> MNPVKREIHPDAVFYKEHKLRNDGLVITTNQGNIRLQFKSEAAIEVLYRADSKQLPSFALAQPESAIKAQLTETENHLQFSGGTLTARIQKRPFAISYYRDSELLLAEESGFQVNTDKINFRFYLSPGEKILGGGQRILGMDRRGQRFPLYNRAHYGYSDHSGQMYFGLPAIMSSKQYILVFDNSASGAMDIGKTESDILQLEAKSGRSAYILVAGNSYPSLIENFTQVTGRQPLPPRWALGSFASRFGYRSEAETRATVQKYKTEDFPLDTIVLDLYWFGKDIKGHMGNLDWDKENFPTPLDMMADFKQQGVKTVLITEPFVLTSSKRWDDAVKAKALAKDPQGQPKAFELYFGNGGIIDVFSKEGSRWFSSIYKDLSKQGVAGWWGDLGEPEMHPEDTQHAIGDADTVHNAYGHRWAEMLYQQQLDQFPELRPFIMMRAGFVGSQRYGMIPWTGDVSRTWGGLASQVELALQMSLLGFGYIHSDLGGFADGETLDKEMYIRWLQYGVFQPVYRPHGQDHIPSEPVFQDEE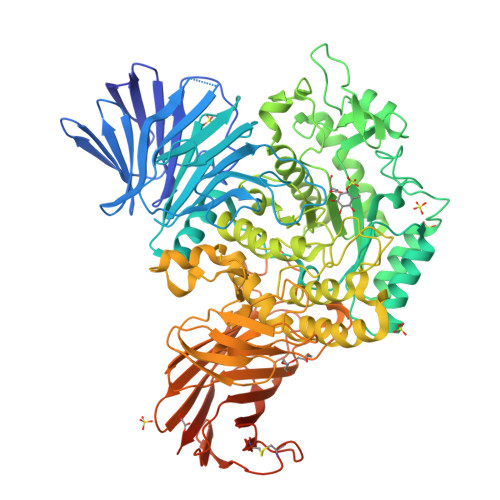TKAILRPLVKLRYRMLPYIYTAAYQNTLTGMPLMRPLFFSDEKNPALIDNKTSYFWGDSLLVTPITQAGVESVSIPAPKGVWFDFWKDTRYQTDGAPLTLPTDLHTIPVLVKAGAFMPYVPAVSTTEDYRSDSLEIHYYADASVPLAQGEIFEDDGKDPNSIKRNQFDLLTLQATHTDNQLHFQLARTGKGYRGMPERRATTLVIHNASDQYQHLDINGKTIAIAQADCASTPALACYDQERRQLQLVFTWGREALNLRLHKGGRADPAFLYKVVINSKLEGKPIPNPLLGLDSTRTGHHHHHH> ETGQCRIQKCTTDFVSLTSHLNSAVDGFDSEFCKALRAYAGCTQRTSKACRGNLVYHSAVLGISDLMS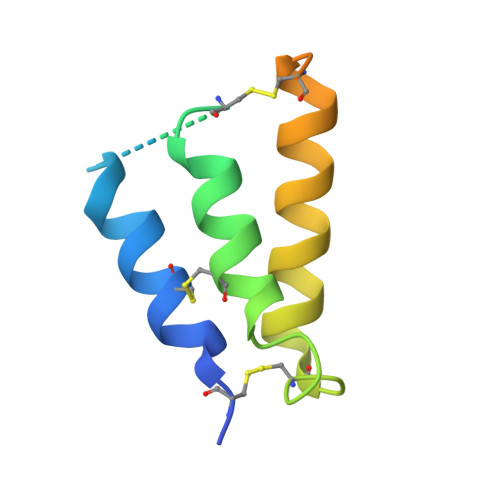QRNCSKDGPTSSTNPEVTHGTKHHHHHH> SEILACEPGGPPPHVPRRSKLVKSPAYGAFPVTKEPAVLSRHDRRTEADVDQVAFSAAGGGDIDEPWPSLIPAVKLYFSRCNFPPLHTLTMLEAINGTPLLDGIDMNQSAGYPWCLTLNRRSLFDVGEDGLYHPCPELYQEIEACLHNPDYFYTTFLKDELRGVDKVAAAKTRLIEAAPIHAIIAGRMLFGGLFEAMHSQPGMYGSAVGCDPDYHWTPFYHSFLDYSEVWALDYSNFDSTIPSVVFKLIGEELAKIIQLPPSIPPDAVQKYVQSIYLSKHVFGDQWYIMKGGNPSGCVGTSILNSMVNNISLLSAMLTHPDFDTS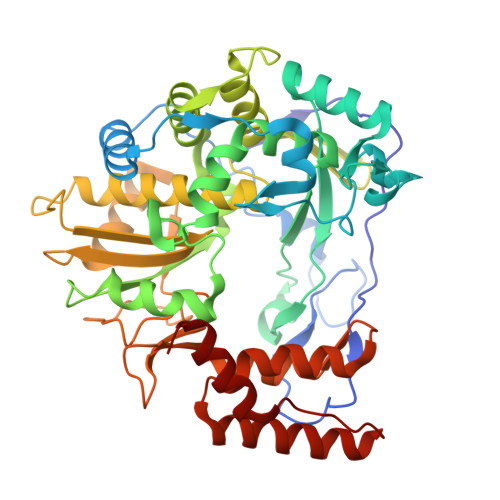AWRILCYGDDVLYATVPSIHPSFIADFYHSQTNYKVTPADKASTFPETSSIHDVTFLKRHFVPDERFPTYIHPVISPETYQQSVMWTRGGPFQDVITSLCYLAHHAGPNNYQKWCDTVQAQCLKSGFEPIFIPYEVLQYRWLATVMT(4R)-6-(1-tert-butyl-1H-pyrazol-4-yl)-4-methyl-1,3,4,5-tetrahydro-2H-1,5-benzodiazepin-2-one | C17 H22 N4 O | 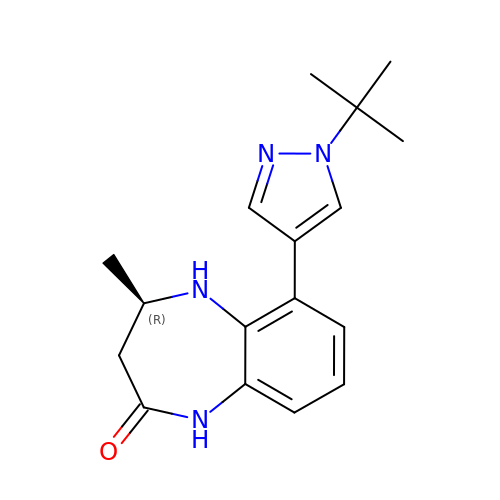HPSNXSAYALRMQW-LLVKDONJSA-N2-imino,3-carboxy,5-hydroxy,6-oxo hexanoic acid | 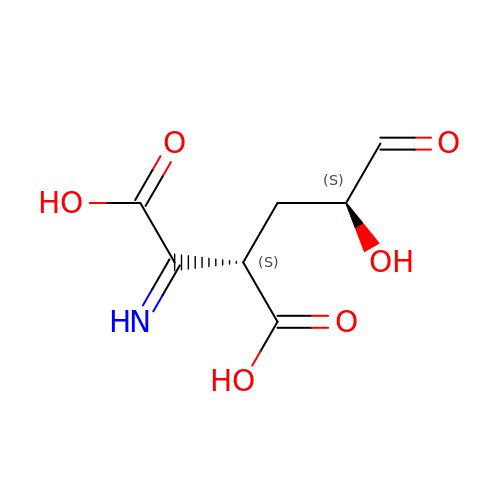C7 H9 N O6 | VTUFCOFLPXRECR-HFOCJQNASA-N Rofecoxib 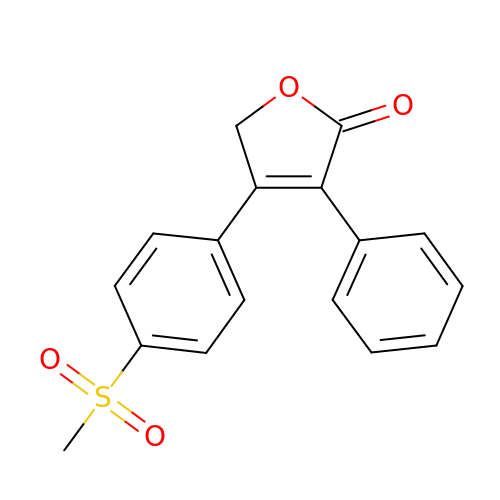| C17 H14 O4 S | RZJQGNCSTQAWON-UHFFFAOYSA-N> MSPITREERLERRIQDLYANDPQFAAAKPATAITAAIERPGLPLPQIIETVMTGYADRPALAQRSVEFVTDAGTGHTTLRLLPHFETISYGELWDRISALADVLSTEQTVKPGDRVCLLGFNSVDYATIDMTLARLGAVAVPLQTSAAITQLQPIVAETQPTMIAASVDALADATELALSGQTATRVLVFDHHRQVDAHRAAVESARERLAGSAVVETLAEAIARGDVPRGASAGSAPGTDVSDDSLALLIYTSGSTGAPKGAMYPRRNVATFWRKRTWFEGGYEPSITLNFMPMSHVMGRQILYGTLCNGGTAYFVAKSDLSTLFEDLALVRPTELTFVPRVWDMVFDEFQSEVDRRLVDGADRVALEAQVKAEIRN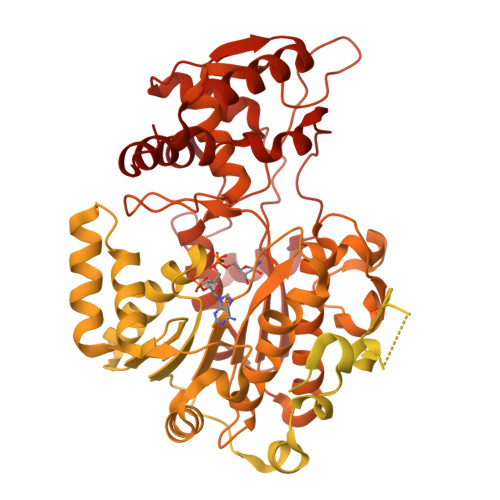DVLGGRYTSALTGSAPISDEMKAWVEELLDMHLVEGYGSTEAGMILIDGAIRRPAVLDYKLVDVPDLGYFLTDRPHPRGELLVKTDSLFPGYYQRAEVTADVFDADGFYRTGDIMAEVGPEQFVYLDRRNNVLKLSQGEFVTVSKLEAVFGDSPLVRQIYIYGNSARAYLLAVIVPTQEALDAVPVEELKARLGDSLQEVAKAAGLQSYEIPRDFIIETTPWTLENGLLTGIRKLARPQLKKHYGELLEQIYTDLAHGQADELRSLRQSGADAPVLVTVCRAAAALLGGSASDVQPDAHFTDLGGDSLSALSFTNLLHEIFDIEVPVGVIVSPANDLQALADYVEAARKPGSSRPTFASVHGASNGQVTEVHAGDLSLDKFIDAATLAEAPRLPAANTQVRTVLLTGATGFLGRYLALEWLERMDLVDGKLICLVRAKSDTEARARLDKTFDSGDPELLAHYRALAGDHLEVLAGDKGEADLGLDRQTWQRLADTVDLIVDPAALVNHVLPYSQLFGPNALGTAELLRLALTSKIKPYSYTSTIGVADQIPPSAFTEDADIRVISATRAVDDSYANGYSNSKWAGEVLLREAHDLCGLPVAVFRCDMILADTTWAGQLNVPDMFTRMILSLAATGIAPGSFYELAADGARQRAHYDGLPVEFIAEAISTLGAQSQDGFHTYHVMNPYDDGIGLDEFVDWLNESGCPIQRIADYGDWLQRFETALRALPDRQRHSSLLPLLHNYRQPERPVRGSIAPTDRFRAAVQEAKIGPDKDIPHVGAPIIVKYVSDLRLLGLL>[2x]DYKDDDDKVLGLKYEEIDCLINDEHTIKGRREGNEVFLPFTWVEKYFDVYGKVVQYDGYDRFEFSHSYSKVYAQRAPYHPDGVFMSFEGYNVEVRDRVKCISGVEGVPLSTQWGPQGYFYPIQIAQYGLSHYSKNLTEKPPHIEVYETAEDRDKNKPNDWTVPKGCFMANVADKSRFTNVKQFIAPETSEGVSLQLGNTKDFIISFDLKFLTNGSVSVVLETTEKNQLFTIHYVSNAQLIAFKERDIYYGIGPRTSWSTVTRDLVTDLRKGVGLSNTKAVKPTKIMPKKVVRLIAKGKGFLDNITISTTAHMAAFFAASDWLVRNQDEKGGWPIMVTRKLGEGFKSLEPGWYSAMAQGQAISTLV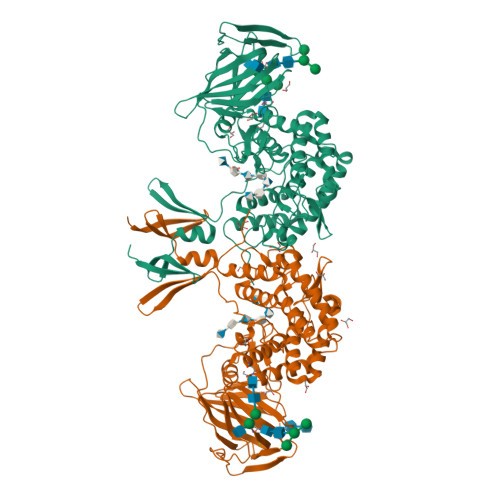RAYLLTKDHIFLNSALRATAPYKFLSEQHGVKAVFMNKHDWYEEYPTTPSSFVLNGFMYSLIGLYDLKETAGEKLGKEARSLYERGMESLKAMLPLYDTGSGTIYDLRHFMLGIAPNLARWDFHTTHINQLQLLSTIDESPVFKEFVKRWKSYLKGSRAKHN>KCTKNALAQTGFNKDKYFNGDVWYVTDYLDLEPDDVPKRYCAALAAGTASGKLKEALYHYDPKTQDTFYDVSELQEESPGKYTANFKKVEKNGNVKVDVTSGNYYTFTVMYADDSSALIHTCLHKGNKDLGD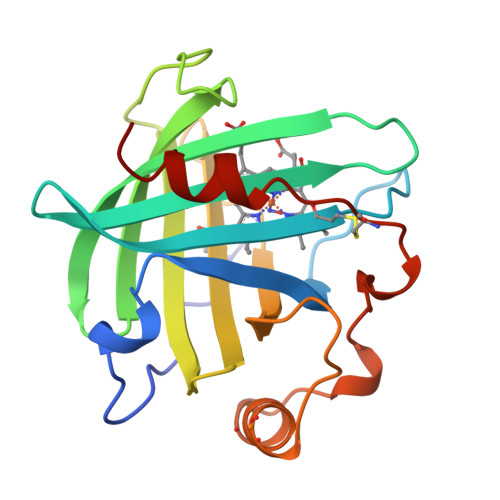LYAVLNRNKDTNAGDKVKGAVTAASLKFSDFISTKDNKCEYDNVSLKSLLTK[2x]(1P)-[1,1'-biphenyl]-3,3'-diol | C12 H10 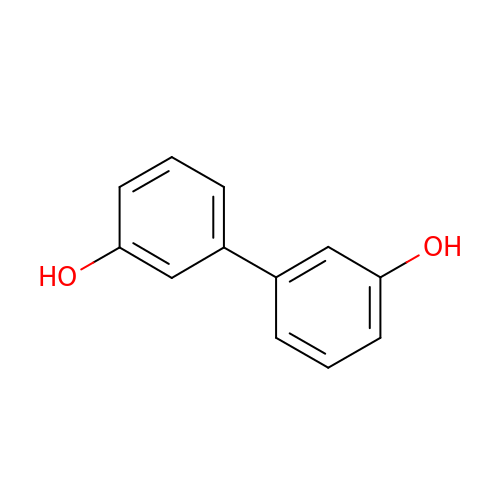O2 | VZQSBJKDSWXLKX-UHFFFAOYSA-N> MKNVYLPITVDHIARVEGKGGVEIVVGDDGVKEVKLNIIEGPRFFEAITLGKKLDEALAIYPRICSFCSAAHKLTAVEAAEKAIGFTPREEIQALREVLYIGDMIESHALHLYLLVLPDYLGYSGPLHMIDEYKKEMSIALDLKNLGSWMMDELGSRAIHQENAVLGGFGKLPDKSVLENMKRRLKEALPKAEYTFELFTKLEQYEEVEGPITHIAVKPRNGVYGIYGDYLKASDGNEFPSEEYREHIKEFVVEHSFAKHSHYHGKPFMVGAISRLVNNADTLYGRAKELYESYKD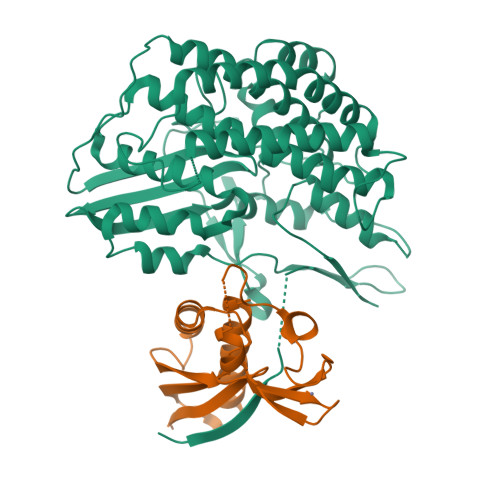LLRSTNPFANNLAQALELVYFTERAIDLIDEALAKWPIRPRDEVALKDGFGVSTTEAPRGVLVYALKVENGRVSYADIITPTAFNLAMMEQHVRMMAEKHYNDDPEKLKLLAEMVVRAYDPCISCSVHVARL;> MHEWALADAIVRTVLDYAQREGASRVKAVRVVLGELQDVAEDIVKFAMEQLFAGTIAEGAEIEFVEEEAVFKCRNCNYEWKLKEVKDKFDERIKEDIHFIPEVVHAFLACPKCGSHDFEVVKGRGVYVAGIKIEKEGGS>TMVLLPNRPAPEFKGQAVINGEFKEICLKDYRGKYVVLFFYPADFTFVPPTEIIAFSDQVEEFNSRNCQVIACSTDSQYSHLAWDNLDRKSGGLGHMKIPLLADRKQEISKAYGVFDEEDGNAFRGLFIIDPNGILRQITI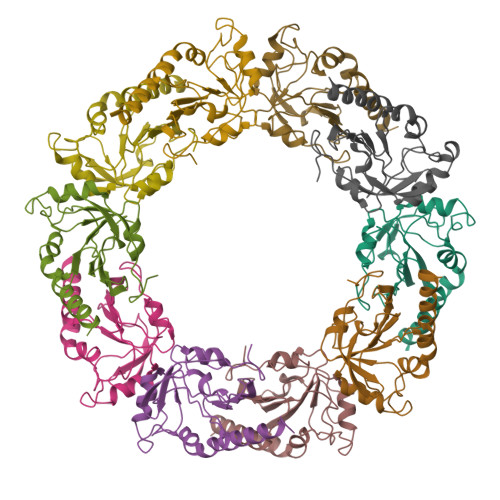NDKPVGRSVDETLRLLDAFQFVEKHGEVCPVNWKRGQHGIKVNQK[40x]>GPLGSASLFATITGASKTEWSFSDIELTYRPNTLLSLGVMEFTLPSGFTANTKDTMNGNALRTTQILNNGKTVRVPLALDLLGAGEFKLKLNNKTLPAAGTYTFRAENKSLSIGNKFYAEASIDVAKRST[9x];> GPLGSASLFATITGASKTEWSFSDIELTYRPDTLLSLGVMEFTLPSGFTANTKDTMNG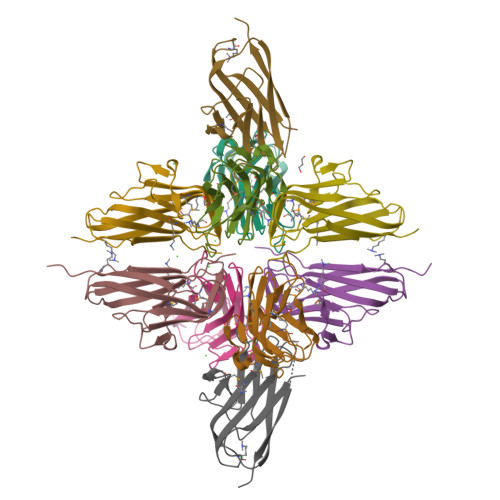NALRTTQILNNGKTVRVPLALDLLGAGEFKLKLNNKTLPAAGTYTFRAENKSLSIGNKFYAEASIDVAKRST> XVDAAVAKVCGSEAIKANLRRSWGVLSADIEATGLMLMSNLFTLRPDTKTYFTRLGDVQKGKAN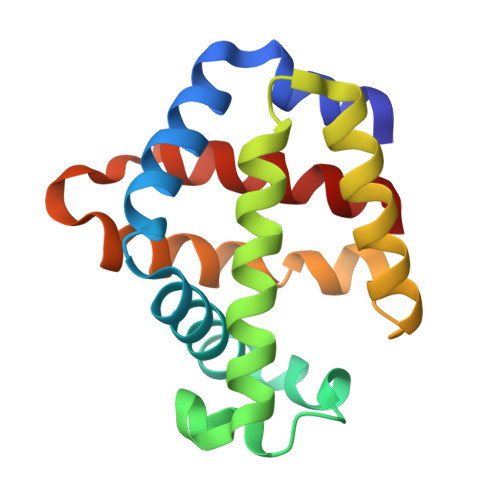SKLRGHAITLTYALNNFVDSLDDPSRLKCVVEKFAVNHINRKISGDAFGAIVEPMKETLKARMGNYYSDDVAGAWAALVGVVQAAL> DVSTSYLRHNEINEYLQTLSQKYPSLVSVEEAGTSYEGRSIKTITINKKPGNAVVFLDAGIHAREWIAPATALYAIEQLVEHSSENQEVLSNLTWVIMPVVNPDGYEFSHETDRFWRKTRKPTGKSCKGTDGNRNFDYHWGEVGASTQACADTFRGETAFSEPETRAVRDAVMKLKGSCKFYLSLHSYGNYILYPWGWTSKLPETWEAIDEVAQAGAEAIKQSTGS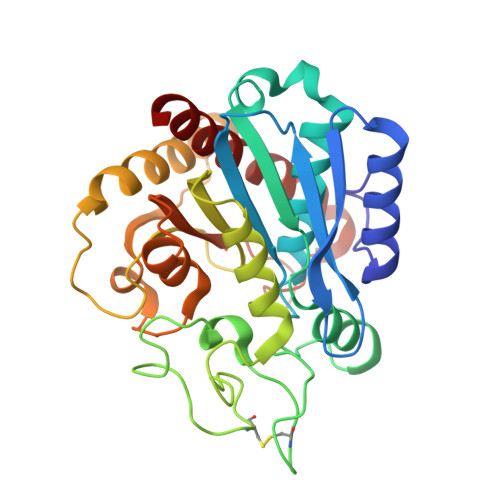RYTVGSSTNVLYAAAGGSDDWAFAVAEVPISITMELPGGGNGGFNPPPSSIEKIVNESWVGIKAMALKVAQMF~{N}-[2-[[(2~{S})-2-[[2,3-bis(oxidanyl)phenyl]carbonylamino]-3-[[(2~{S})-2-[[2,3-bis(oxidanyl)phenyl]carbonylamino]-3-oxidanylidene-3-(prop-2-ynylamino)propyl]amino]-3-oxidanylidene-propyl]amino]-2-oxidanylidene-ethyl]-2,3-bis(oxidanyl)benzamide 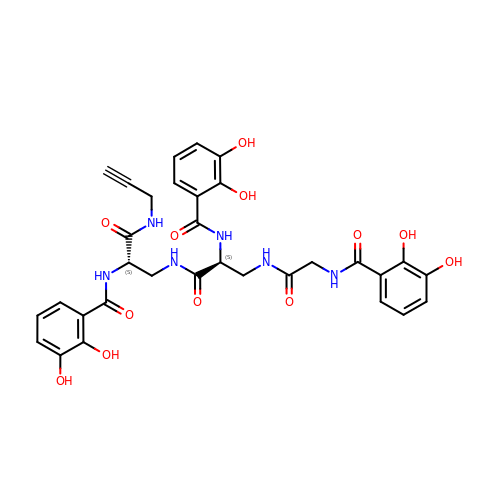| C32 H32 N6 O12 | XJMZSRWAQFOMTB-PMACEKPBSA-N>[6x]AEIYNKDGNKVDLYGKAVGLHYFSKGNGENSYGGNGDMTYARLGFKGETQINSDLTGYGQWEYNFQGNNSEGADAQTGNKTRLAFAGLKYADVGSFDYGRNYGVVYDALGYTDMLPEFGGDTAYSDDFFVGRVGGVA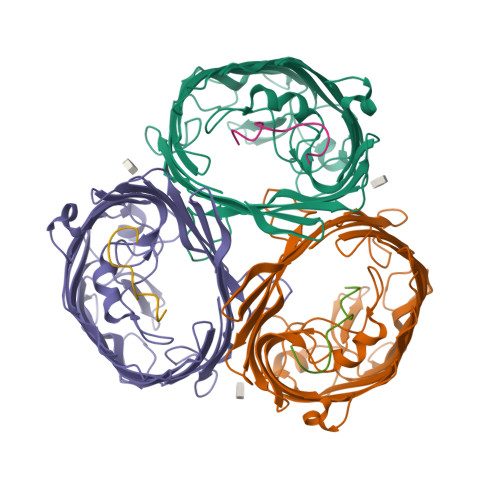TYRNSNFFGLVDGLNFAVQYLGKNERDTARRSNGDGVGGSISYEYEGFGIVGAYGAADRTNLQEAQPLGNGKKAEQWATGLKYDANNIYLAANYGETRNATPITNKFTNTSGFANKTQDVLLVAQYQFDFGLRPSIAYTKSKAKDVEGIGDVDLVNYFEVGATYYFNKNMSTYVDYIINQIDSDNKLGVGSDDTVAVGIVYQF;>SGGDGRGHNTGAHSTSG[6x]> MIVPVLSRQALRHASVARVALPSLTRWYASYPPHTVVKMPALSPTMTSGGIGAWQKKPGDKIEPGEVLVEIETDKAQMDFEFQEEGVLAKILKDSGEKDVAVGNPIAILVEEGTDVNAFKDFTLKDAGGETSPAVPKDEPKNESTASAPTPAPTPAPEPENTSFTGRFQTALEREPNALPAAKRLAREKGIDLRNVKGSGPGGKITEEDVKKALASAPAAGAAAAAYTDVPISGMRKTIAAR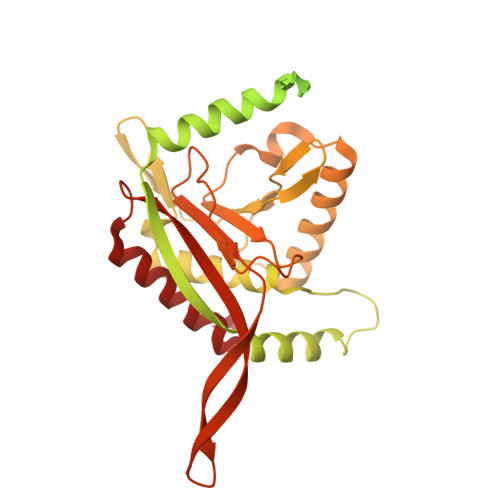LKESVTENPHFFVSTNLSVSKLLKLRQALNSSADGRYKLSVNDFLIKAMGIASKRVPTVNSSWRDGVIRQFETVDVSVAVATPNGLITPIVKGVEGKGLESISAAVKELAKKARDGKLKPEEYQGGSISISNMGMNPAVQSFTAIINPPQAAILAVGAPQKVAVPVENEDGTTGVSWDEQIIVTASFDHKVVDGAVGAEWIRELKKVIENPLELLL>[2x]GSQSPEEDRIIVSNCLYEQLKDKARLIAQSDHFSFIAIPIDENITNTLQKMRPVCGNYLNAEPYIQQTSNRFLDSKKLLDKLTSYHSISTANPYPINHEAQV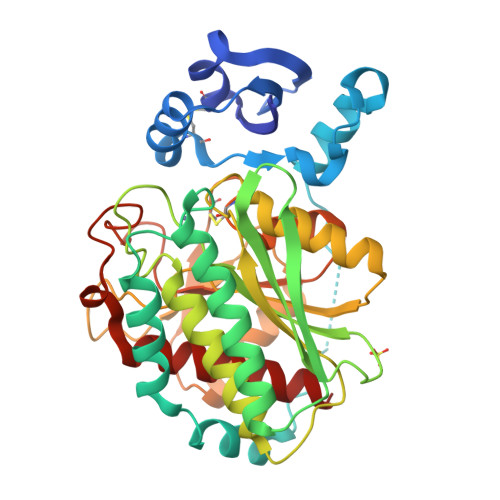HSLFEQIDPAKIWQTNQHLTSYINRSAKSRTGVEAAQWFKQQFDTLAQDYGRKDVESYFVKTGNKFIQPSVVTVIGKDKPGEAIVIGAHIDTLDGNMPGADDDSSGISVELEMARVVFSSNFELNRPIYFIAYAAEERGLIGSGYVVQDFLQKKIPVKAVMQLDQAGYRANAKDQTIWLLKDYVDKGLTEFTAELLTRYVKTPVGYTKCGYACSDHVNWTNEGFKTTYPSATTLDDDNPYVHTSNDTLDILNLEHMVNFTKLGLAFIVELGLN> PVTTSFWRIATDARTYEADDLSGAGAKITGGRWNEVGVAIVYAASSRAMACLETVVHLNSGGLPLNRYLVEIEVPDEVLASAEVATPGNLPVGWDAEPAGRV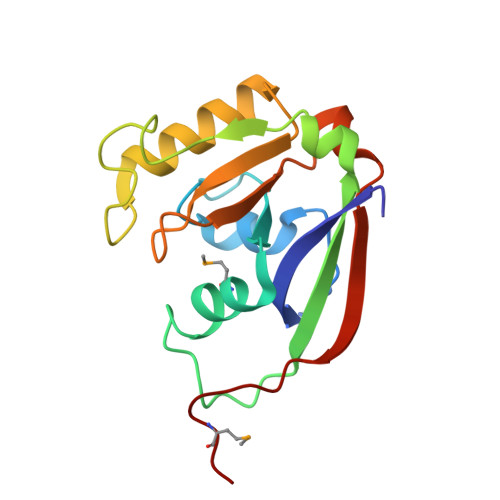SISFGSQWAQSQRTALLLVPSVIVPEETNLLINPAHPDAKGIKARKVRKWLYDPRMIR>MTSQEKSMPFIKHLASSDRKVRTAALNSLHAFLSARQVASALTTLDVLKLWKGLFYALWMCDRAIPQQNLCNELADLIWQLPRESVATWLRGFWATMAREWTGIDVLRMEKFLLLVRRVLGASFKWMKKDGSLGKRTHDGQEKAVKTGAWDQSKVDEVLGLLAEWPFSLAEEVRITQSSEKGGEIVQKIPVGMRLHVLDIWVDEVERVGLLNEDEEEARMIVQRISDMVDALEQTTKSPAVRTRSKDSLGDDRLPANRRPNSS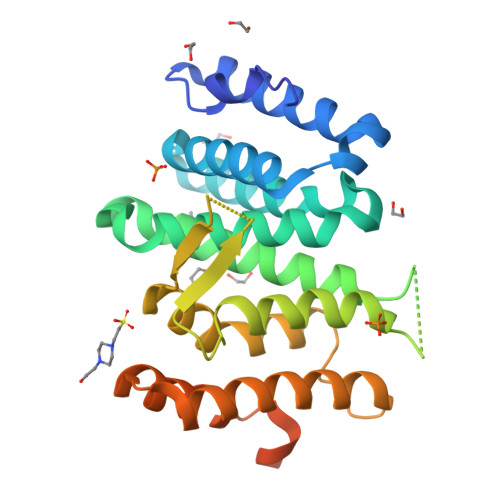QDHDTKDMGDSDSWEGFDDGSHHHHHH[2x]> DESQVPDQPSSLHVRPQTNCIIMSWTPPLNPNIVVRGYIIGYGVGSPYAETVRVDSKQRYYSIERLESSSHYVISLKAFNN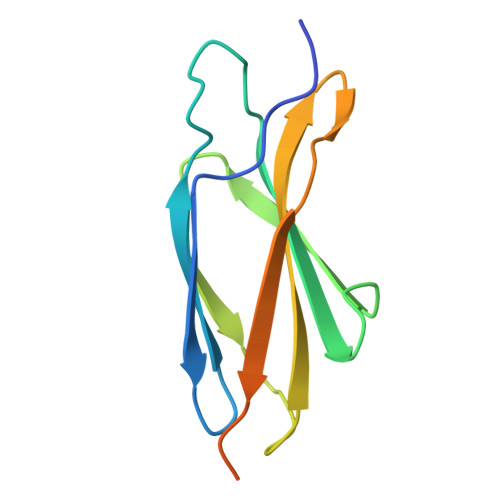AGEGVPLYESATTRGSGGSGGSGGSGGSGGSGGSG> SLSSTQSVNSVLAPGNLRKVHHIALNVQDMQASRYFYGTILGLHELTDDEVPATLTELVASGKVANFITPDGTILDLFGEPELSPPDPNPEKTFTRAYHLAFDIDPQLFDRAVTVIGENKIAIAHGPVTRPTGRGVYFYDPDGFMIEIRCDPEA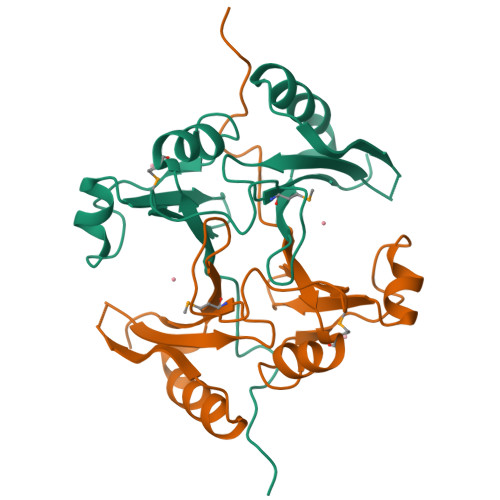EG>MAPAEILNGKEISAQIRARLKNQVTQLKEQVPGFTPRLAILQVGNRDDSNLYINVKLKAAEEIGIKATHIKLPRTTTESEVMKYITSLNEDSTVHGFLVQLPLDSENSINTEEVINAIAPEKDVDGLTSINAGRLARGDLNDCFIPCTPKGCLELIKETGVPIAGRHAVVVGRSKIVGAPMHDLLLWNNATVTTCHSKTAHLDEEVNKGDILVVATGQPEMVKGEWIKPGAIVIDCGINYVPDDKKPNGRKVVGDVAYDEAKERASFITPVPGGVGPM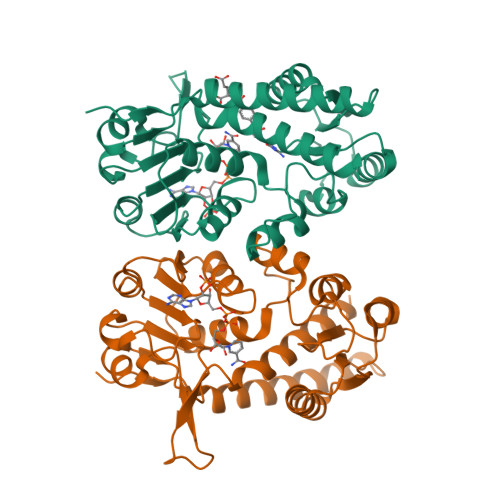TVAMLMQSTVESAKRFLE[2x]> MTLRAAVFDLDGVLALPAVFGVLGRTEEALALPRGLLNDAFQKGGPEGATTRLMKGEITLSQWIPLMEENCRKCSETAKVCLPKNFSIKEIFDKAISARKINRPMLQAALMLRKKGFTTAILTNTWLDDRAERDGLAQLMCELKMHFDFLIESCQVGMVKPEPQIYKFLLDTLKASPSEVVFLDDIGANLKPARDLGMVTILVQDTDTALKELEKVTGIQLLNTPAPLPTSCNPSDMSHGYVTVKPRVRLHFVELGSGPAVCLCHGFPESW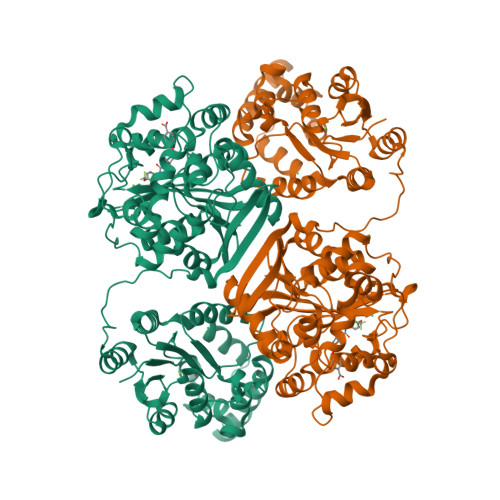YSWRYQIPALAQAGYRVLAMDMKGYGESSAPPEIEEYCMEVLCKEMVTFLDKLGLSQAVFIGHDWGGMLVWYMALFYPERVRAVASLNTPFIPANPNMSPLESIKANPVFDYQLYFQEPGVAEAELEQNLSRTFKSLFRASDESVLSMHKVCEAGGLFVNSPEEPSLSRMVTEEEIQFYVQQFKKSGFRGPLNWYRNMERNWKWACKSLGRKILIPALMVTAEKDFVLVPQMSQHMEDWIPHLKRGHIEDCGHWTQMDKPTEVNQILIKWLDSDARNPPVVSKM>[2x]AGRFAQSQTREDYLALLAE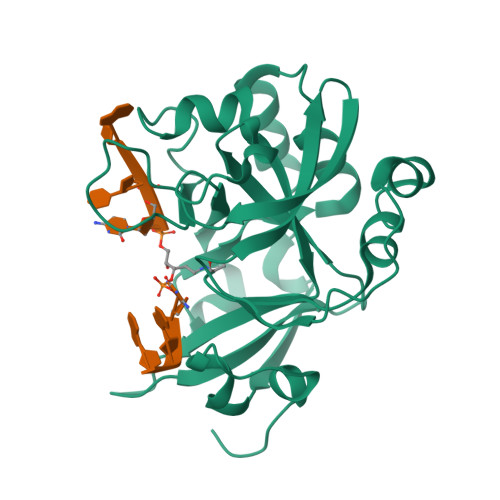DIERDIPYDPEPIGRYNVAPGTKVLLLSERDEHLHLDPVFWGYAPGWWDKPPLINARVETAATSRMFKPLWQHGRAICFADGWFEWKKEGDKKQPFFIYRADGQPIFMAAIGSTPFERGDEAEGFLIVTAAADQGLVDIHDRRPLVLSPEAAREWMRQEISGKEASEIAASGCVPANQFSWHPVSRAVGNVKNQGAELIQPVLEVLFQ>VPATLPQLTPTLVSLLEVIEPEVLYAGYDSSVPDSTWRIMTTLNMLGGRQVIAAVKWAKAIPGFRNLHLDDQMTLLQYSWMYLMAFALGWRSYRQSSANLLCFAPDLIINEQRMTLPGMYDQCKHMLYVSSELHRLQVSYEEYLCMKTLLLLSSVPKDGLKSQELFDEIRMTYIKELGKAIVKREGNSSQNWQRFYQLTKLLDSMHEVVE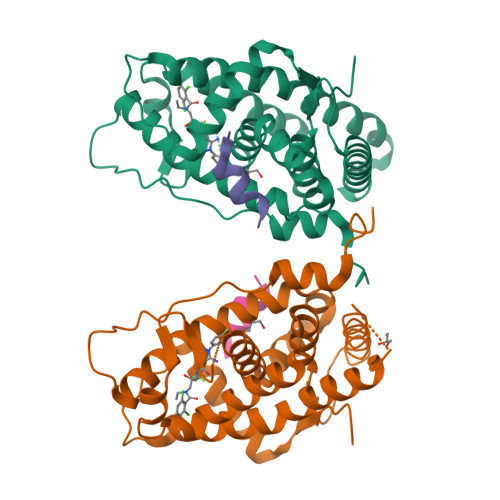NLLNYCFQTFLDKTMSIEFPEMLAEIITNQIPKYSNGNIKKLLFHQK[2x];>ENALLRYLLDK[2x]4-[3-[[2,6-bis(azanyl)-5-(3-chlorophenyl)pyrimidin-4-yl]methoxy]phenoxy]butanoic 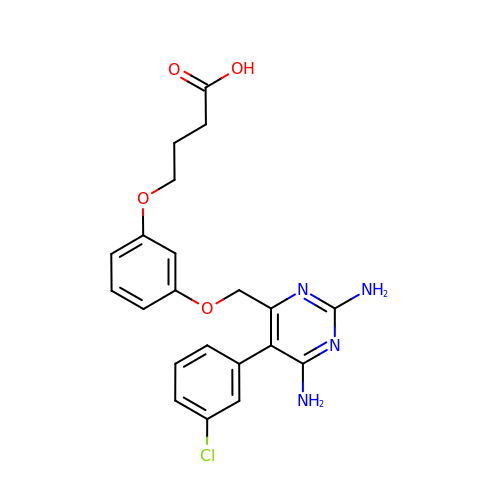acid | C21 H21 Cl N4 O4 | CSFKBCPKDXDYEY-UHFFFAOYSA-N> GSPGLDGICQSTSNHLWLLSDILGQGATANVFRGRHKKTGDLYAVKVFNNISFLRPVDVQMREFEVLKKLNHKNIVKLFAIEEETTTRHKVLIMEFCPCGSLYTVLEEPSNAYGLPESEFLIVLRDVVGGMNHLRENGIVHRDIKPGNIMRVIGEDGQSVYKLTDFGAARELEDDEQFVALYGTEEYLHPDMYERAVLRKDHQKKYGATVDLWSVGVTFYHAATGSLPFRPFEGPRRNKEVMYKIITGKPSGAISGVQKAENGPIDWSGDMPLSCSLSQGLQALLTPVLANILEADQEKCWGFDQFFAETSDVLHRMVIHVFSLQHMTAHKIYIHSYNTAAVFHELVYKQTKIVSSNQELIYEGRRLVLELGRLAQHFPKTTEENPIFVTSREQLNTVGLRYEKISLPKIHPRYDLDGDASMAKA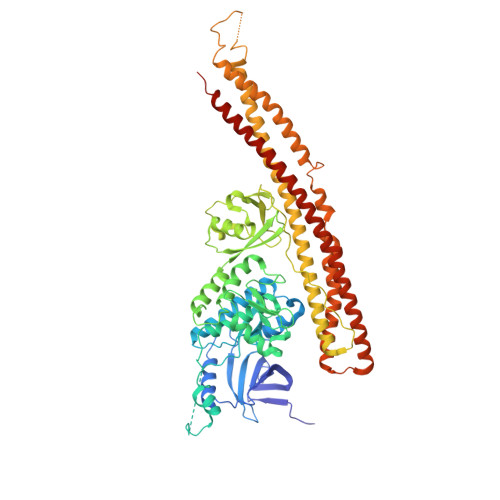VTGVVCYACRTASTLLLYQELMRKGVRWLVELVKDDYNETVHKKTEVVITLDFCIRNIEKTVKVYEKLMKVNLEAAELGEISDIHTKLLRLSSSQGTIESSLQDISSRLSPGGLLADTWAHQEGTHPRDRNVEKLQVLLNCITEIYYQFKKDKAERRLAYNEEQIHKFDKQKLYYHATKAMSHFSEECVRKYEAFKDKSEEWMRKMLHLRKQLLSLTNQCFDIEEEVSKYQDYTNELQET The T4S system of H. pylori translocates the major effector protein CagA into gastric epithelial cells. As an essential component of the cagPAI T4S system core complex, CagX plays a critical role in CagA translocation into the host cell. CagX is presumed to be structurally and functionally homologous to VirB9 from the well studied VirB/D4 T4S of the plant pathogen Agrobacterium tumefaciens, although the two proteins have low sequence identity. Here, we report the expression, purification, crystallization, structure determination and analysis of the C-terminal domain of the CagX protein (CagXct).

The CagXct crystal structure was solved by MR and subjected to isotropic B-factor twin refinement in REFMAC5 at 1.4 Å resolution after the true space group had been established as monoclinic P21 with a β angle close to 90°, with the crystal forming a nonmerohedral twin. It contains two protein monomers with all residues built into the electron density, one PEG and two 2-propanol molecules and 129 waters. The two monomers of CagXct comprising the asymmetric unit can be superimposed with an r.m.s.d. of 0.38 Å over all 103 Cα atoms. To maintain structural similarity, many buried protein residues which form the protein core of TraO are conserved or substituted by residues with similar properties in CagX. Most amino-acid residues of strand β1, which runs antiparallel to TraN in TraO, are not conserved in CagX; however, the main chains of the matching residues of both these T4S proteins have the same conformation and solvent accessibility. Thus, it appears likely that the β-sheet interaction between TraO and TraN is reproduced in the Cag–CagT interface. Interestingly, one of the 2-propanol molecules binds to the main-chain N atom of the Ramachandran plot outlier Asp481 in monomer A in the CagXct structure. The main-chain N atom of the equivalent Gly258 in TraO forms a hydrogen bond to the main-chain O atom of Gly364 in TraF, with the positions of Gly364 and the 2-propanol ligand O atoms overlapping.

>[2x]PVPRNYNYYQAPEKRSKHIMPSEIFDDGTFTYFGFKNITLQPAIFVVQPDGKLSMTDAAIDPNMTNSGLRWYRVNEIAEKFKLIKDKALVTVINKGYGKNPLT>HMGSMALDGIRMPDGCYADGTWELSVHVTDLNRDVTLRVTGEVHIGGVMLKLVEKLDVKKDWSDHALWWEKKRTWLLKTHWTLDKCGIQADAKLQFTPQHKLLRLQLPNMKYVKVKVNFSDRVFKAVSDICKTFNIRHPEELSLLKKPRDPTKKKKKKLDDQSEDEALELEPGILAVSQPVTSPEILAKMFKPQALLDKAKTNQGWLDSSRSLMEQDVKENEALLLRFKYYSFFDLNPKYDAIRINQLYEQAKWALLLEEIECTEEEMMMFAALQYHINKLSIMTSENHLTTDVNPECLVSPRYLKKYKSKQITARILEAHQNVAQMSLIEAKMRFIQAWQSLPEFGITHFIARFQGGKREELIGIAYNRLIRMDASTGDAIKTWRFSNMKQWNVNWEIKMVTVEFADEVRLSFICTEVDCKVVHEFIG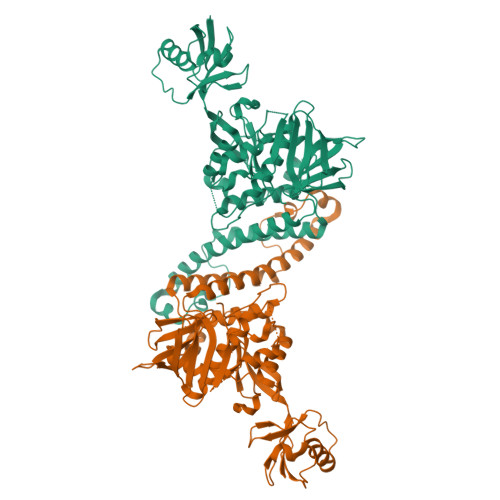GYIFLSTRAKDQNESLDEEMFYKLTSGWVLVPRGSGSGSGSKEATSTFTNITYRGT[2x]>INPKFKDLRAYYTKPSLEFKNEIGIILKKWTTIRFMNVVPDYFIYKIALVGKDDKKYGEGVHRNVDVFVVLEENNYNLEKYSVGGITKSNSKKVDHKAGVRITKEDNKGTISHDVSEFKITKEQISLKE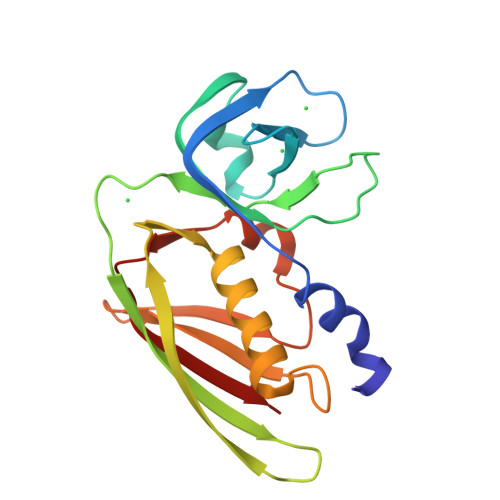LDFKLRKQLIEKNNLYGNVGSGKIVIKMKNGGKYTFELHKKLQENRMADVIDGTNIDNIEVNIK[2x]>GPDEEPEEPGRRGSFVEMVDNLRGKSGQGYYVEMTVGSPPQTLNILVDTGSSNFAVGAAPHPFLHRYYQRQLSSTYRDLRKGVYVPYTQGKWEGELGTDLVSIPHGPNVTVRANIAAITESDKFFINGSNWEGILGLAYAEIARPDDSLEPFFDSLVKQTHVPNLFSLQLCGAGFPLNQSEVLASVGGSMIIGGIDHSLYTGSLWYTPIRREWYYEVIIVRVEINGQDLKMDCKEYNYDKSIVDSGTTNLRLPKKVFEAAVKSIKAASSTEKFPDGFWLGEQLVCWQAGTTPWNIFPVISLYLMGEVTNQSFRITILPQQYLRPVEDVATSQDDCYKFAISQSSTGTVMGAVIMEGFYVVFDRA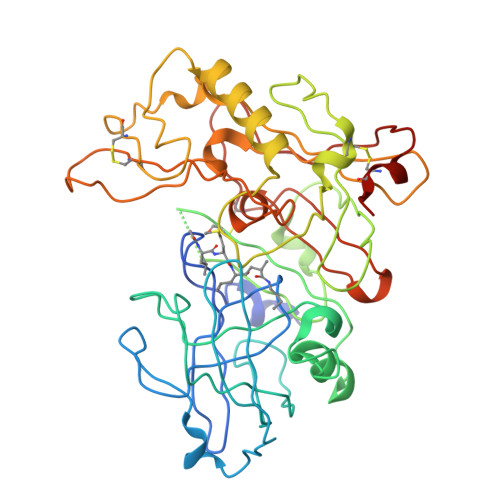RKRIGFAVSACHVHDEFRTAAVEGPFVTLDMEDCGYNIPQTDES[3x]> VPPAIVVLIGPPGYVGKQYPITASDIVIGRSVESQVYIDDKSLSRSHAKFAVNGSEVSVIDLGSTNKTIVNGQVIPPLASCLLKNNDQ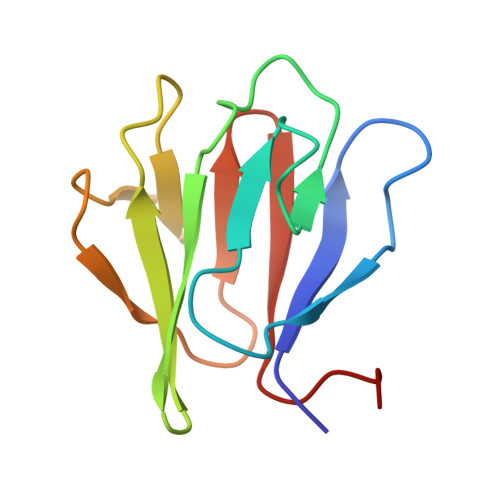IKTGNVIFKFLEKGSIE> MNILLVSQCEKRALSETRRILDQFAERRGERTWQTPITQAGLDTLRRLLKKSARRNTAVACHWIRGRDHSELLWIVGDASRFNAQGAVPTNRTCRDILRKEDENDWHSAEDIRLLTVMAALFHDIGKASQAFQAKLRNRGKPMADAYRHEWVSLRLFEAFVGPGSSDEDWLRRLADKRETGDAWLSQLARDDRQSAPPGPFQKSRLPPLAQAVGWLIVSHHRLPNGDHRGSASLARLPAPIQSQWCGARDADAKEKAACWQFPHGLPFASAHWRARTALCAQSMLERPGLLARGPALLHDSYVMHVSRLILMLADHHYSSLPADSRLGDPNFPLHANTDRDSGKLKQRLDEHLLGVALHSRKLAGTLPRLERQLPRLARHKGFTRRVEQPRFRWQDKAYDCAMACREQAMEHGFFGLNLASTGCGKTLANGRILYALADPQRGARFSIALGLRSLTLQTGQAYRERLGLGDDDLAILVGGSAARELFEKQQERLERSGSESAQELLAENSHVHFAGTLEDGPLREWLGRNSAGNRLLQAPILACTIDHLMP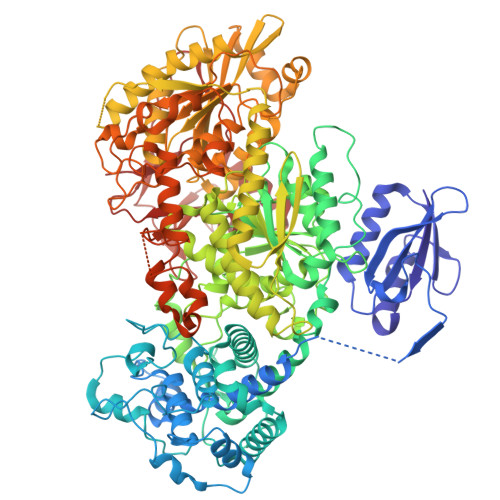ASESLRGGHQIAPLLRLMTSDLVLDEVDDFDIDDLPALSRLVHWAGLFGSRVLLSSATLPPALVQGLFEAYRSGREIFQRHRGAPGRATEIRCAWFDEFSSQSSAHGAVTSFSEAHATFVAQRLAKLEQLPPRRQAQLCTVHAAGEARPALCRELAGQMNTWMADLHRCHHTEHQGRRISFGLLRLANIEPLIELAQAILAQGAPEGLHVHLCVYHSRHPLLVRSAIERQLDELLKRSDDDAAALFARPTLAKALQASTERDHLFVVLASPVAEVGRDHDYDWAIVEPSSMRSIIQLAGRIRRHRSGFSGEANLYLLSRNIRSLEGQNPAFQRPGFETPDFPLDSHDLHDLLDPALLARIDASPRIVEPFPLFPRSRLVDLEHRRLRALMLADDPPSSLLGVPLWWQTPASLSGALQTSQPFRAGAKERCYALLPDEDDEERLHFSRYEEGTWSNQDNLLRNLDLTYGPRIQTWGTVNYREELVAMAGREDLDLRQCAMRYGEVRLRENTQGWSYHPYLGFKKYN> DGVPAVVDCDVHAVLPSPHSLIPYLDEYWADQLVAQLAPTYEPNYHPRGSAIAQHSDASVDENGRAATTAENLVKDVFADGFTDFAVVNCLYGVQQIHQPRREMAHARALNHWIANEWLDKDDRLRASIVVPQGSPRAAAEEIDFWSGDKRFVQVLLLGQSELLYGREINWPIWEAAEAAGLPVTLHIGGVFRQAPTSVGWPASHLEWYVGQQSNIEAQLNSIISEGILQKFPKTKILLSELGFNWLPPFMWKFDKLWKSYRPDIPWVQESPLELIREHVRVTTSPS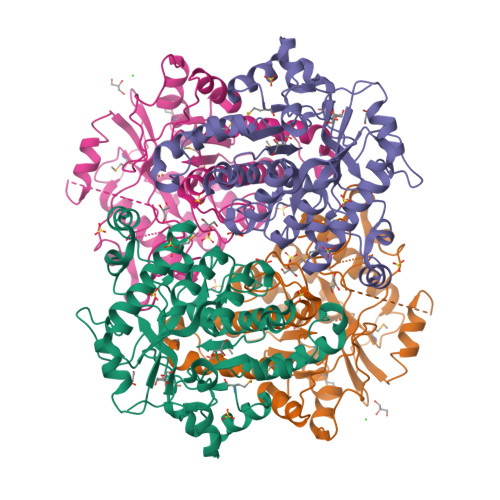DGAEEAGRLDSIVDRLGSDRMLVYSSDYPHKHHSGPRDIENGTHSPELLDRIYRRNAFDLYNLVVPS;> MTIIEHGSLGTLPAPSVTTGIVDADIHPVPQDGALEPYLDDRWKKHIREYGVRTTTGLQFISEYPQMYGGAMRADAWPESGYPGSDRELLRTQLLDKHNIQLGVLQCLAPGGQTLNPAGQALNQELAAALCRATNDWQLEHLVYPDPRMRAAIPVTFETPDYAVAEIERVGADPGVVAVLGTSKTLEPLGSRKYWPIYEASVAQNLPIQFHLSQGGGHANTGTGWTSYHTEYHTGHVQSFQSQLLSLVLSGTFDRFPTLKVMFVEGNVAHFAPLIQRMDYTWETLRGELPDLQRKPSEYIRDHIWASTQPIDEPEKPEHLAELLEEFCGDNVVFATDYPHFDFDDPETAFPRSFPVDLRDKILRGNGMRFFGVTNQAD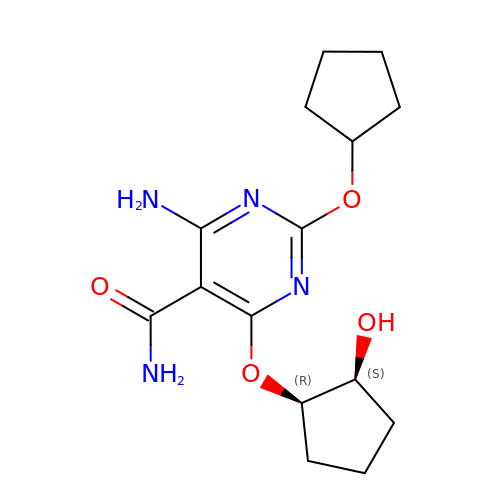4-amino-2-(cyclopentyloxy)-6-{[(1R,2S)-2-hydroxycyclopentyl]oxy}pyrimidine-5-carboxamide | C15 H22 N4 O4 | GOYBCUMANOWCAY-VHSXEESVSA-N1-AMINOCYCLOPROPYLPHOSPHONATE | C3 H7 N O3 P | 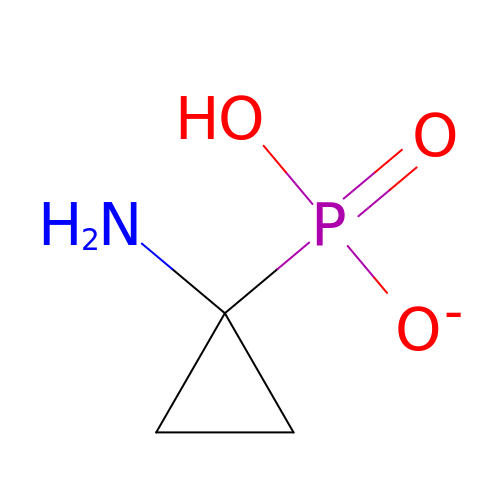WKCJTSHOKDLADL-UHFFFAOYSA-M>GAMETLHITKTMKNIEVPETKTASFECEVSHFNVPSMWLKNGVEIEMSEKFKIVVQGKLHQLIIMNTSTEDSAEYTFVCGNDQVSATLTVT[16x]

Evidence accumulated over the past two decades has identified titin as a main coordinator of cardiac muscle homeostasis, and its dysfunction through genetic mutation as an important factor in cardiomyopathy. For this, we examined the unique mSNP T2850I in the I-band domain of titin I10, as a paradigm of an alteration in a general component of the titin chain. Domain I10 does not support specific interactions or have any known specialized roles, so it does not constitute an a priori sensitive locus of the chain. In previous studies, we have shown that the T2580I mSNP destabilizes the affected immunoglobulin (Ig) domain in titin, I10, and speculated that this instability increases the vulnerability of titin to proteolysis in situ potentially leading to myocardial damage.

We calculated a total of 17 molecular copies of I10 originating from two different space groups and diverse non-crystallographic symmetries. The structural features of all 17 molecular copies of I10 were in strict agreement (global RMSD = 0.62 Å for 82 matched Cα atoms across all models, calculated using MUSTANG). T2850 is stabilized in this conformation by two hydrogen bonds: (i) a short, strong bond (2.4 Å) between its side chain hydroxyl and the carbonyl of the previous residue, E2849, and (ii) a second contact between its main chain amide group and the main chain carbonyl of T2897 in the neighbouring EF loop. The side chain hydrogen bond turns the otherwise atomic clash into a productive interaction and permits T2850 to adopt a high-energy conformation within the generously allowed αL Ramachandran region. When mapped onto the crystal structure of I10, the perturbations largely clustered around the mutation site, in the A'B β-turn and the neighbouring EF loop that are interconnected through hydrogen bonds mediated by T2850. This shows that the mutation only introduces modest local distortions in the I10-fold. The large difference in measured thermal stability was difficult to understand, as the exchange involves the removal of a single hydrogen bond (established by the Thr side chain with the main chain of the preceding residue; T2850-OH:CO-E2849) in the otherwise-intact fold.> GSHMASNKYKRIFLVVMDSVGIGEAPDAEQFGDLGSDTIGHIAEHMNGLQMPNMVKLGLGNIREMKGISKVEKPLGYYTKMQEKSTGKDTMTGHWEIMGLYIDTPFQVFPEGFPKELLDELEEKTGRKIIGNKPASGTEILDELGQEQMETGSLIVYTSADSVLQIAAHEEVVPLDELYKICKIARELTLDEKYMVGRVIARPFVGEPGNF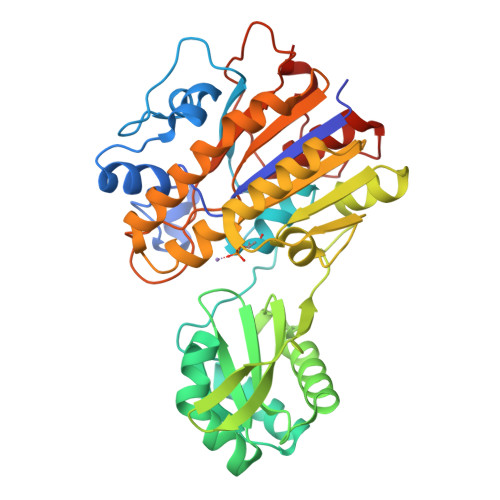TRTPNRHDYALKPFGRTVMNELKDSDYDVIAIGKISDIYDGEGVTESLRTKSNMDGMDKLVDTLNMDFTGLSFLNLVDFDALFGHRRDPQGYGEALQEYDARLPEVFAKLKEDDLLLITADHGNDPIHPGTDHTREYVPLLAYSPSMKEGGQELPLRQTFADIGATVAENFGVKMPEYGTSFLNELKK Base excision repair (BER) is the pathway primarily tasked with repairing DNA base damage, with apurinic/apyrimidinic endonuclease (APE1) having both AP-endonuclease and 3′ to 5′ exonuclease (exo) DNA cleavage functions. Importantly, 3′-8-oxoG impairs the ligation step of BER and therefore must be removed by the exo activity of a surrogate enzyme to prevent double stranded breaks and cell death. APE1 has been shown to be the major 3′-exonuclease activity responsible for the repair of 3′-8-oxoG lesions in human cells. APE1 end processing of 8-oxoG, during which the oxidative DNA lesion is removed, results in a ‘clean’ 1-nt gapped substrate suitable for DNA synthesis by Pol β during BER.

To see how the APE1 active site accommodates 3′-8-oxoG, we crystallized APE1 bound with nicked, double stranded DNA substrates containing 8-oxoG at the 3′-end and a phosphate at the 5′-end of the SSB. These substrates represent potentially unligatable, BER intermediates in which the repair polymerase, Pol β, has misinserted an 8-oxodGTP across from either a templating A or C. To obtain crystals of the substrate complexes, we employed a double-mutant catalytically dead variant of APE1 (E96Q/D210N). Specifically, DNA bending at the site of the nick results in an open intra-helical cavity in the DNA, and in both cases the 8-oxoG base is in an anti-conformation and positioned out of the protein active site into the open intra-helical cavity where it does not form any base-pairing interactions with the opposing A or C. This conformation allows the damage-containing 3′ end of the DNA nick and phosphate backbone to shift into the protein active site for cleavage. Of note, density for the 8-oxoG base is relatively weak, for the structure with 8-oxoG opposite C. We attempted, but were unable to obtain, crystals of APE1 with an analogous uncleavable (i.e. phosphothioate containing) substrate. Therefore, it is likely that the relatively weak density for the 8-oxoG base is the result of high mobility, as opposed to low occupancy. Supporting this, the B-factors for the 3′-8-oxoG, as well as the 5′-base and opposing base, are higher in the case of 8-oxoG opposite C. This high mobility in the DNA region around and including the 3′-8-oxoG base likely results from the lack of WC base paring between the 3′-8-oxoG base and the opposing base and the open active site pocket in which the 8-oxoG nucleobase resides. A similar phenomenon occurs with the N210 substitution, which coordinates OD1 of N68, thus resulting in ND2 coordinating the nucleophilic water molecule. Similar contacts occur between the APE1 protein side chains and the phosphate backbone of 3′-8-oxoG opposite C, Figure 4C. Specifically, the hydrogen bonding between R177 (NH2) and the 8-oxoG O6 oxygen atom is weaker, 3.0 versus 2.6 Å, in the case of the O8:C structure due to the contact between R177 and C requiring R177A to shift further towards the opposing strand than when it is opposite A.

>ALYEDPPDQKTSPSGKPATLKICSWNVDGLRAWIKKKGLDWVKEEAPDILCLQQTKCSENKLPAELQELPGLSHQYWSAPSDKEGYSGVGLLSRQAPLKVSYGIGDEEHDQEGRVIVAEFDSFVLVTAYVPNAGRGLVRLEYRQRWDEAFRKFLKGLASRKPLVLCGNLNVAHEEIDLRNPKGNKKNAGFTPQERQGFGELLQAVPLADSFRHLYPNTPYAYTFWTYMMNARSKNVGWRLDYFLLSHSLLPALCDSKIRSKALGSDHCPITLYLAL[2x]>GCKDNDDATGDFDPNKPVVISEFSPKEGGLGTRMLLYGENFGSDISKIKVTIGGQDSKVVGAKGKSLYCVVPAKAYDGDIKLSILNDEGEEIANTEANEKFVYQKKMLVTTFLGTMYDGNTKYDLKDGPFDDCGGFGGAVWLSFDPKNHNHLYLVGEQHPTRLIDFEKEYVSTVYSGLSKVRTICWTHEADSMIITNDQNNNDRPNNYILTRESGFKVITELTKGQNCNGAETHPINGELYFNSWNAGQVFRYDFTTQETTPLFTIQDSGWEFHIQFHPSGNYAYIVVVNQHYILRSDY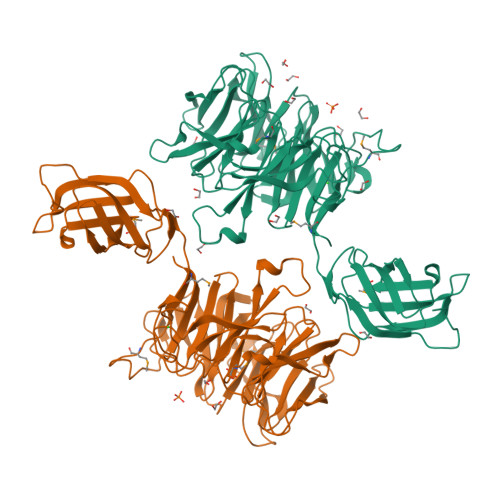DWKTKRLTTPYIVCGQQGAKDWVDGVGKKARMHAPRQGTFVKNPAYKGSSDEYDFYFCDRENHCIRILTPQGRVTTFAGRGSNGTSGYNDGDLRQEARFNHPEGIVYDEERECFFIGDRENRRIRKIGYEE[2x]3-oxidanyl-2-[3,5,6-tris(chloranyl)-4-[(4-chlorophenyl)methylamino]pyridin-2-yl]carbonyl-cyclohex-2-en-1-one 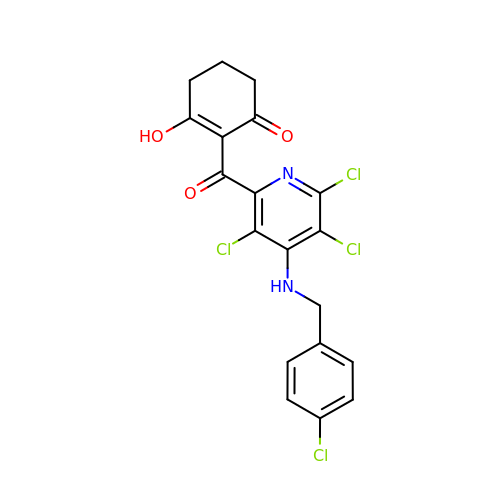| C19 H14 Cl4 N2 O3 | MQJYIBCWAJRDCH-UHFFFAOYSA-N>[3x]AYSNTYQEFTNIDQAKAWGNAQYKKYGLSKSEKEAIVSYTKSASEINGKLRQNKGVINGFPSNLIKQVELLDKSFNKMKT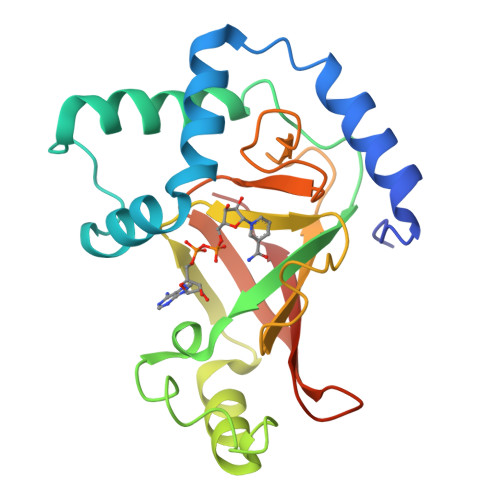PENIMLFRGDDPAYLGTEFQNTLLNSNGTINKTAFEKAKAKFLNKDRLEYGYISTSLMNVSQFAGRPIITKFKVAKGSKAGYIDPISAFAGQLNMLLPRHSTYHIDDMRLSSDGKQIIITATMMGTAINPK> KQGIVKSDPKLPDDTTFPLPPPRPKNVIFEDEEKSKMLARLLKSSHPEDLRAANKLIKEMVQEDQKRMEKISKRVNAIEEVNNNVKLLTEMVMSHSQGGAAAGSSEDLMKELYQRCERMRPTLFRLASDTEDNDEALAEILQANDNLTQVINLYKQLVRGEEV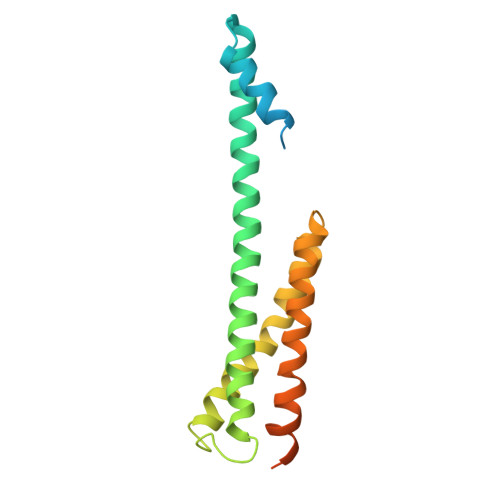NGDATAGSIPGSTSALLDLSGLD>[2x]DKLASGRSVVSCPANCLCASNILSCSKQQLPNVPQSLPSYTALLDLSHNNLSRLRAEWTPTRLTNLHSLLLSHNHLNFISSEAFVPVPNL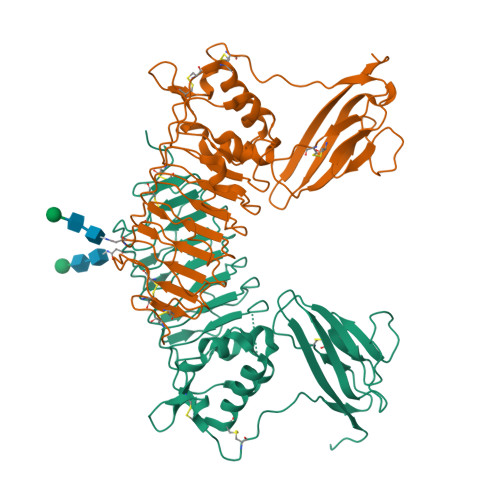RYLDLSSNHLHTLDEFLFSDLQALEVLLLYNNHIVVVDRNAFEDMAQLQKLYLSQNQISRFPVELIKDGNKLPKLMLLDLSSNKLKKLPLTDLQKLPAWVKNGLYLHNNPLECDCKLYQLFSHWQYRQLSSVMDFQEDLYCMHSKKLHNIFSLDFFNCSEYKESAWEAHLGDTLTIRCDTKQQGMTKVWVSPSNEQVLSQGSNGSVSVRNGDLFFKKVQVEDGGVYTCYAMGETFNETLSVELKVYNFTLHGHHDTLNAAADPWSHPQFEK>[2x]MSRQSISLRFPLLLLLLSPSPVFSADPGAPAPVNPCCYYPCQHQGICVRFGLDRYQCDCTRTGYSGPNCTIPEIWTWLRTTLRPSPSFIHFLLTHGRWLWDFVNATFIRDTLMRLVLTVRSNLIPSPPTYNIAHDYISWESFSNVSYYTRILPSVPRDCPTPMDTKGKKQLPDAEFLSRRFLLRRKFIPDPQSTNLMFAFFAQHFTHQFFKTSGKMGPGFTKALGHGVDLGHIYGDNLERQYQLRLFKDGKLKYQMLNGEVYPPSVEEAPVLMHYPRGIPPQSQMAVGQEVFGLLPGLMLYATIWLREHNRVCDLLKAEHPTWGDEQLFQTARLILIGETIKIVIEEYVQQLSG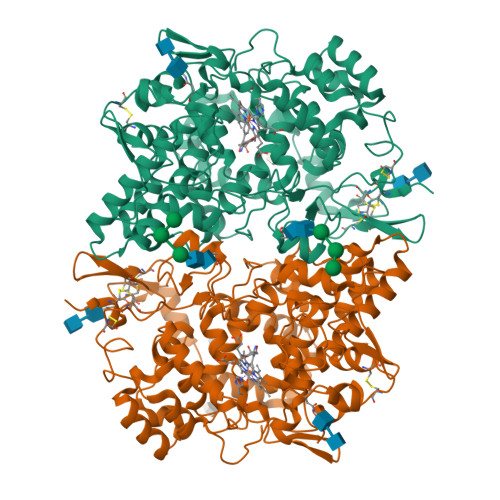YFLQLKFDPELLFGAQFQYRNRIAMEFNQLYHWHPLMPDSFRVGPQDYSYEQFLFNTSMLVDYGVEALVDAFSRQPAGRIGGGRNIDHHILHVAVDVIKESRVLRLQPFNEYRKRFGMKPYTSFQELTGEKEMAAELEELYGDIDALEFYPGLLLEKCHPNSIFGESMIEMGAPFSLKGLLGNPICSPEYWKASTFGGEVGFNLVKTATLKKLVCLNTKTCPYVSFHVPDPRQEDRPGVERPPTEL>LYFQGHMTAEVRRDSFKTFWDKYSDKPDTNSMMLNQTAQDLEASDRADILSSLPHLTNKDVVDIGAGIGRFTTVLAETARWVLSTDFIESFIEKNQERNAHMGNISYQIGDAVHLQMDEKSVDLVFTNWLMMYLSDREVIEFLLNAMRWLRADGYIHLRESCSEPSTGRLKTATMHSAVDANPTHYRFSSLYIKLLRAIRYRDSDGKMWKFDVQWSCSVPTYIRRCNNWRQVHWLTKKVPAVGDEETSVDDLLNLFSQIWPAEQKTWDEKLDNEKYSWTDKIFSNAIDDEVVPKNSTAYVFTPRQRSPFLHVNSHLLAEKFTCNVWNVETKEYLYRTSLTKANNQKDQRVRFGWNESLSSSIDYWNQRDASFDCMVA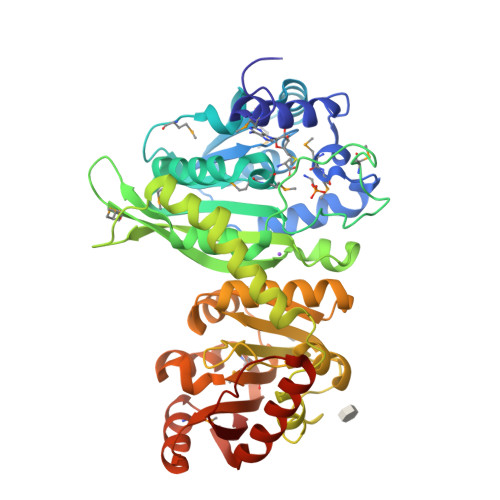TELLATCDDESINSIASIMKPEAKVVLLEPVSGIDETSVRQRMTTCGFKNITIVDVTQESLNAEVSFIKDHNLDVELSGCNYLLIKASL[2x]> GPLGSMDSSQLHVAIVSSPGMGHLIPVLVLGNRLATHHNIKITILAITTTSSSAETEFLKKTTLTNEEKTIEIIPVPSVDISHLINSSTKIFTQLRLLVREALPKIHSTIASMTHRPDALIVDIFCTQILPIAEEFNISKYTYHPTTAWTLALAIYCQVFDKEIEGEYVELKEPLKIPGCKALRPDDVVDPLLDRSDQQYEEYVKLGKEYTDFDGILINTWEDLEPETINALRYNEKLRLLLKVPVFPIGPLRRKVETTLNDEVIQWLDKQNNESVLFVSFGSGGTLSTKQMTELAWGLELSQQKFVWVVRPPSDGDADSAYLNSAGKDTRDMSEYLPEGFLTRTKDMGLVVPMWANQVEILSHSSVGGFLTHCGWNSTVESLTNGVPMIAWPLHAEQKMNAAMLTEELGVAIRPAVLPTKKLVKREEIQGMVRILMQTKEGKRIKEKAKKLKKSAENALSDGGSSYNSICELVKDIRSREL

NbUGT72AY1 is a promiscuous transferase that glycosylates bioactive hydroxycoumarins such as scopoletin and umbelliferone, as well as monolignols involved in lignin formation and various other small molecules. Five distinct GT protein folds have been identified that are capable of GT activity (termed GT-A to GT-E). NbUGT72AY1 adopts a GT-B fold comprised of two distinct N-terminal and C-terminal Rossmann-like domains (shown in cyan and brown in Fig. 2, respectively) of seven and six parallel β-sheets, respectively linked to α-helices, connected by a linker region and an interdomain cleft. The catalytic mechanism of inverting UGT such as NbUGT72AY1 is a direct displacement bimolecular nucleophilic substitution (SN2)-like reaction enabled by an enzymatic base catalyst.

To gain insight into the mechanism of NbUGT72AY1 catalysis, SI and UDPG glucohydrolase activity, we determined the crystal structure of the monomeric protein (apo) and complexes revealing the structural alterations induced by different ligands such as scopoletin (acceptor), UDP (product), UDP-2-deoxy-2-fluoro-D-glucose (UDP2FG, donor substitute), β-carotene (effector), retinol (effector) and combinations thereof. In addition to the apo-form (I), a protein structure was obtained, which crystallized in β-carotene-containing solution (II), differed from the apo-form, and lacked the electron density for the ligand. Asn372, Ser373, Glu376, Arg249, Ala351, and Trp350 frame their donor binding sites and in both structures, the indole ring of Trp350 points in the direction towards the uracil structure of UDP2FG and UDP, resulting in a π-stacking interaction. All other complexes that vary in their bound ligands have one (III, VI, VII, VIII, and IX) or two (I and II) disordered sequence parts (shown as red sticks in Fig. 2) located between Ile42-Leu59 and Ser309-Asp327. Upon substrate binding, the disordered Ile42-Leu59 sequence part in the apo-protein transforms into helix H2, which aligns parallel to helix H1 above the catalytic site. Starting with the apo-enzyme (I), two different conformational changes can occur after substrate binding depending on whether the acceptor (I → III) or donor (I → VII) is the first to interact with the protein. Thus, as the crystal structures indicate, random binding of substrates to the apo-enzyme is possible, but the products are formed only after ordered sequential binding of the substrates.>[2x]GSHMGSKSSAAKEGAGAVDEEDFIKAFDDVPVVQIYSSRDLEESINKIREILSDDKHDWEQRVNALKKIRSLLLAGAAEYDNFFQHLRLLDGAFKLSAKDLRSQVVREACITLGHLSSVLGNKFDHGAEAIMPTIFNLIPNSAKIMATSGVVAVRLIIRHTHIPRLIPVITSNCTSKSVAVRRRCFEFLDLLLQEWQTHSLERHISVLAETIKKGIHDADSEARIEARKCYWGFHSHFSREAEHLYHTLESSYQKALQSHLKNSDSIVSLPQS

Two prime animal MAP families that bind tubulin and are recruited to microtubule plus ends by EB proteins (either directly or indirectly) are the Cytoplasmic Linker-Associated Protein (CLASP) family and the XMAP215 family of microtubule polymerases. While XMAP215 family members promote microtubule polymerization, CLASP family members promote microtubule pause, potentiate rescue, and limit catastrophe. While the CLASP and XMAP215 families differentially affect microtubule dynamics, they both employ an array of tubulin-binding TOG domains to regulate the microtubule polymer. While mammalian XMAP215 family members contain an N-terminal pentameric TOG domain array, mammalian CLASPs contains three TOG domains (TOG1-3) followed by a C-terminal CLIP-170 interaction domain (CLIP-ID).

To determine if this architecture was due to crystal packing, we determined the structure of H.s. CLASP1 TOG2 in a different space group, P21, as compared to the initial structure that was determined in the space group P212121. Native diffraction data was collected to a resolution of 1.78 Å, was 98.1% complete overall, and was 85.4% complete in the 1.84–1.78 Å high-resolution shell with an average I/σI of 2.8 in the high-resolution shell. The crystal contains two protomers in the asymmetric unit. CLASP1 TOG2 is 65 Å in length with a bend between the HR A-C and HR D-F triads that orients the HR D-F intra-HR loop surface at ~30° relative to the plane established by the HR A-C intra-HR loops. This deviates significantly from the flat surface observed across XMAP215 family TOG intra-HR loops used to engage tubulin (discussed further below). Comparing protomers determined in the P21 space group to those determined in the P212121 space group showed little structure deviation with low overall Cα pairwise rmsd values that ranged from 0.3 to 1.3 Å. Collectively, the bent architecture of CLASP family TOG2 domains is conserved and reflects a key structural state of the domain. Of the highly conserved intra-HR loops, most of the conservation is located along the first triad, HR A-C. The HR A loop contains a conserved tryptophan, positioned equivalent to the conserved HR A loop tryptophan found in XMAP215 family TOG domains that engages β-tubulin. CLASP1 TOG2 is curved across the tubulin-binding surface and our structural modeling suggests that it may engage tubulin in a hyper-curved state.2-azanylpenta-1,4-dien-3-one | C5 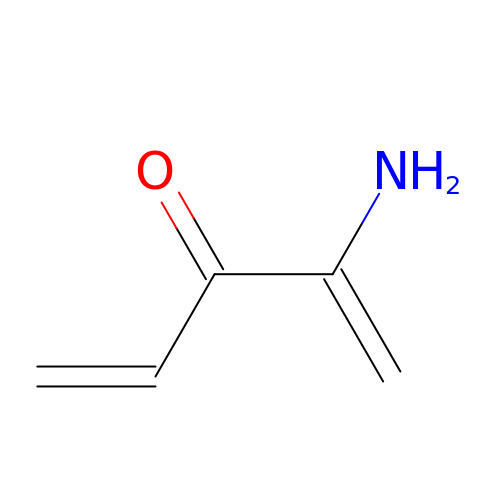H7 N O | AHTXUWSCLWCTPN-UHFFFAOYSA-N> QNSLALHKVI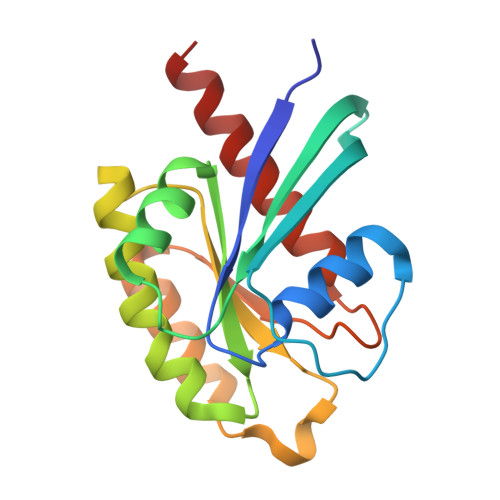MVGSGGVGKSALTLQFMYDEFVEDYEPTKADSYRKKVVLDGEEVQIDILDTAGQEDYAAIRDNYFRSGEGFLCVFSITEMESFAATADFREQILRVKEDENVPFLLVGNKSDLEDKRQVSVEEAKNRAEQWNVNYVETSAKTRANVDKVFFDLMREIRARKMEDS> MADFSLATASQRKEWSNKAHMEYVRRSRFAPYIRNTENSIFQGYSDLEKRAGDTLNIPLFYKLGGAPVTGDTPIVGNETPLDNYNCGVPVALRGKGVAITKNQTFRTEIDVMNAAKQSLTRYFGELLRDDIIEALGSVVTTGDTTVNYGSASAANRNAFSAANPDRLFFGSISGYSATWATGLGNVDAAETCTAARVGVMKRLAMSASPAITPMQVDDDEGREYFVAFHGSRTFRDLKGDTAMLNANREARPRDVSSNPLLQDGDLIYEGVIHREVPEIDAWAAANGFNTAGAGSAPIRPVFLCGTQSVFLAYAQRPQAGTEKS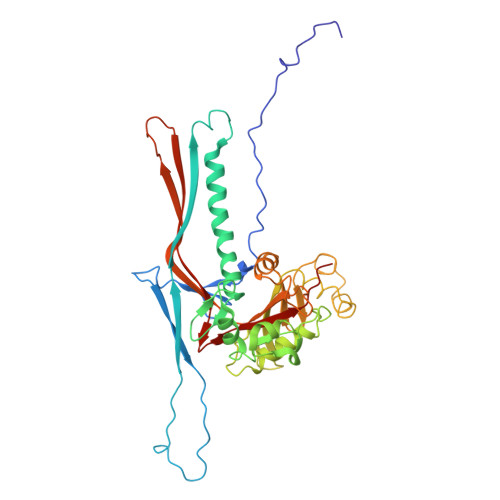DIPALNRRMTVGMDEIIGVKKAAFNGKQHGVVMGFFGAAGD> MSLKKEYLQCQSLVDVVRLRALHSPNKKSCTFLNKELEETMTYEQLDQHAKAIAATLQAEGAKPGDRVLLLFAPGLPLIQAFLGCLYAGCIAVPIYPPAQEKLLDKAQRIVTNSKPVIVLMIADHIKKFTADELNTNPKFLKIPAIALESIELNRSSSWQPTSIKSNDIAFLQYTSGSTMHPKGVMVSHHNLLDNLNKIFTSFHMNDETIIFSWLPPHHDMGLIGCILTPIYGGIQAIMMSPFSFLQNPLSWLKHITKYKATISGSPNFAYDYCVKRIREEK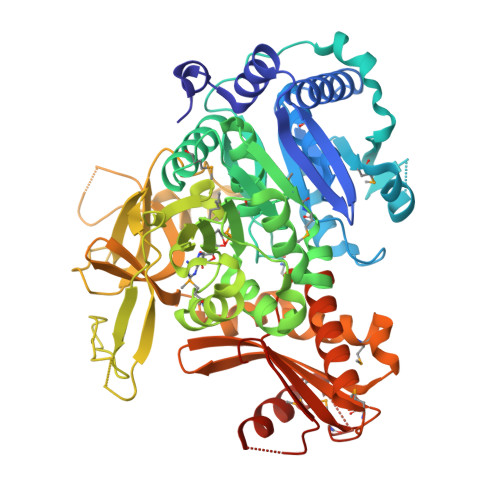KEGLDLSSWVTAFNGAEPVREETMEHFYQAFKEFGFRKEAFYPCYGLAEATLLVTGGTPGSSYKTLTLAKEQFQDHRVHFADDNSPGSYKLVSSGNPIQEVKIIDPDTLIPCDFDQVGEIWVQSNSVAKGYWNQPEETRHAFAGKIKDDERSAIYLRTGDLGFLHENELYVTGRIKDLIIIYGKNHYPQDIEFSLMHSPLHHVLGKCAAFVIQEEHEYKLTVMCEVKNRFMDDVAQDNLFNEIFELVYENHQLEVHTIVLIPLKAMPHTTSGKIRRNFCRKHLLDKTLPIVATWQLNKIEEGHHHHHH>MIGFLTDWGLKSHYVGVAKAVIKRINPSAEIIDITHEVEPFNVRKASHVLYRASLDFPPSTVFLVVVDYGVGTSRKAIVMKTKNDQYFVAPDNGVLTVVAEEYGVAEIREIENRELFYKKNPSFTFHGRDIFAPVAAHLDMGLPLERVGDRLLSYEVLKMRKPVVENEKVIGEVAIVDTFGNVSTNIPFDLFLKLSVDFDDVVRVRVGRKEFKAAV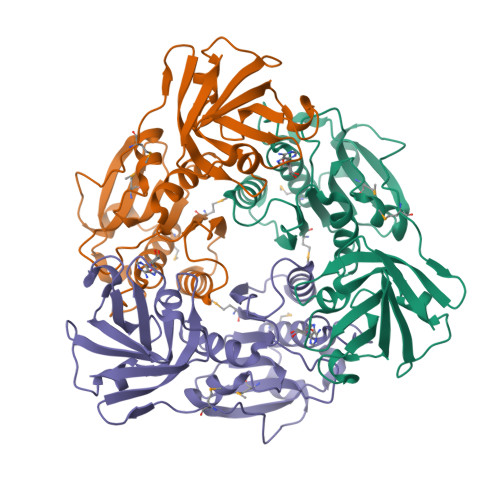AKAFGDVDTGELLVHPDSAGFLEIAVNLGDASQVLSVKEGDEIEICR[4x]>MLCEIECRALSTAHTRLIHDFEPRDALTYLEGKNIFTEDHSELISKMSTRLERIANFLRIYRRQASELGPLIDFFNYNNQSHLADFLEDYIDFAINEPDLLRPVVIAPQFSRQMLDRKLLLGNVPKQMTCYIREYHVDRVIKKLDEMCDLDSFFLFLHGRAGSGKSVIASQALSKSDQLIGINYDSIVWLKDSGTAPKSTFDLFTDILLMLKSEDDLLNFPSVEHVTSVVLKRMICNALIDRPNTLFVFDDVVQEETIRWAQELRLRCLVTTRDVEISNAASQTCEFIEVTSLEIDECYDFLEAYGMPMPVGEKEEDVLNKTIELSSGNPATLMMFFKSCEPKTFEKMAQLNNKLESRGLVGVECITPYSYKSLAMALQRCVEVLSDEDRSALAFAVVMPPGVDIPVKLWSCVIPVDICSNEEEQLDDEVADRLKRLSKRGALLSGKRMPVLTFKIDHIIHMFLKHVVDAQTIANGISILEQRLLEIGNNNVSVPERHIPSHFQKFRRSSASEMYPKTTEETVIRPEDFPKFMQLHQKFYDSLKNFACC[2x];> MMRQDRRSLLERNIMMFSSHLKVDEILEVLIAKQVLNSDNGDMINSCGTVREKRREIVKAVQRRGDVAFDAFYDALRSTGHEGLAEVLEPLARSVDSNAVEFECPMSPASHRRSRALSPAGYTSPTRVHRDSVSSVSSFTSYQDIYSRARSRSRSRALHSSDRHNYSSPPVNAFPSQPSSANSSFTGCSSLGYSSSRNRSFSKASGPTQYIFHEEDMNFVDAPTISRVFDEKTMYRNFSSPRGMCLIINNEHFEQMPTRNGTKADKDNLTNLFRCMGYTVICKDNLTGRGMLLTIRDFAKHESHGDSAILVILSHGEENVIIGVDDIPISTHEIYDLLNAANAPRLANKPKIVFVQACRGERRDNGFPVLDSVDGVPAFLRRGWDNRDGPLFNFLGCVRPQVQQVWRKKPSQADILIAYATTAQYVSWRNSARGSWFIQAVCEVFSTHAKDMDVVELLTEVNKKVACGFQTSQGSNILKQMPEMTSRLLKKFYFWPEARNSAV

In Caenorhabditis elegans (C. elegans), onset of programmed cell death is marked with the activation of CED-3, a process that requires assembly of the CED-4 apoptosome. CED-3 is synthesized as an inactive zymogen; its activation requires association with the CED-4 apoptosome. Activated CED-3 forms a holoenzyme with the CED-4 apoptosome to cleave a wide range of substrates, leading to irreversible cell death. Here, we report cryo-EM structures of the CED-4 apoptosome and three distinct CED-4/CED-3 complexes that mimic different activation stages for CED-3.

We thereby assembled the ternary complex of CED-4/CED-3_CARD/CED-3 catalytic domain, hereafter referred to as the holoenzyme, to mimic the full-length CED-4/CED-3 complex (orange). In the presence of the catalytic domain of CED-3, more than half of CED-4, 52.1% existed as octamers. The octameric CED-4 is nearly identical to that in the crystal structure, with the eight CARDs observing a group I stacking. The ring-like density on the top of the CED-4 apoptosome can be assigned with four CED-3 CARDs. Overall, the tower is of ∼120 Å tall and ∼170 Å wide at the bottom. CARD–CARD interaction between CED-3 and CED-4 involves helices H1 and H4 of CED-3. Basic residues on CED-3, including Arg7, Arg63, and Arg64 appeared to contact the acidic residues on CED-4 CARD, including Asp20, Asn78, and Asn79 (cyan rectangle). Compared with WT CED-3 CARD, less R7D co-migrated with CED-4, whereas R63A/R64A no longer associated with CED-4. In contrast, neither CED-3 R7D nor CED-3 R63A/R64A responded to CED-4 apoptosome, supporting an essential role of the CARD–CARD interaction in CED-3 activation (lane 4–6). However, in the structure of the holoenzyme and the CED-4/CED-3_CARD complex, four CED-3 CARDs were resolved.>GSHMAAAKQDVKVFSEDGTSKVVEILADMTARDLCQLLVYKSHSVDDNSWTLVEHHPHLGLERCLEDHELVVQVESTMASESKFLFRKNYAKYEFFKNPMNFFPEQMVTWSQQSNGSQTQLLQNFLNSSSSPEIQGFLHVKELGKKSWKKLYVCLRRSGLYCSTKGTSAAPRHLQLLADLEDSNIFSLIAGRKQYNAPTDHGLCIKPNKVRNETKELRLLC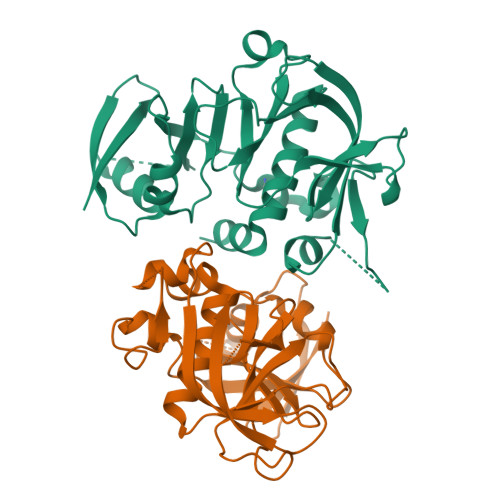AEDEQTRTSWMTAFRLLKYGMLLYQNYRIPQQRKA[2x]ETS1/2, unlike GABPA, only activate −146C>T mutant TERT promoter through cooperation with p52 downstream of non-canonical NF-κB signaling. p52 is a member of the NF-κB family of transcription factors which regulate gene expression in response to a wide array of signaling by binding to consensus κB sites of 5′-GGGRNYYYCC-3′ (R is a purine, Y is a pyrimidine, and N is any nucleotide). The major domains of ETS1 protein include the PNT domain, the acidic transactivation domain, the ETS DNA-binding domain and autoinhibitory module which consists of inhibitory helix 1 (HI1), inhibitory helix 2 (HI2), helix 4 (H4), and helix 5 (H5). p52 consists of the Rel homology domain and the glycine-rich region.

We next determined the crystal structure of p52-RHD (residues 35–329) in complex with ETS1331–441 and a 15 bp DNA fragment of TERT promoter containing −146C>T ETS motif (designated as p52/ETS1/−146C>T). The final refined model contains the 15 bp DNA fragment, p52 residues 226–328 designated as the dimerization subdomain of p52-RHD (p52-DSD), and ETS1 residues 332–437. The DNA-binding subdomain of p52-RHD (p52-DBSD, residues 35–225) is assumed to be disordered as its electron densities are not clear enough for unambiguous model building. H3 inserts into the major groove of the DNA and contacts the GGAA central core specifically. In the p52/ETS1/−146C>T ternary complex structure, ETS1 recognizes the −146C>T TERT promoter exclusively and concurrently interacts with p52-DSD. The interaction of p52 and ETS1 buries a total solvent accessible surface area of 1187 Å2. p52 uses the loops flanking one end of the β-barrel of p52-DSD to interact with α-helices H1, H4, H5, loop H4–H5 and N-terminal region of ETS1 domain predominantly through a network of hydrogen bonds and salt bridge contacts, supplemented with additional van der Waals contacts. Structural superposition of ETS1 in the p52/ETS1/−146C>T complex and the autoinhibited ETS1 showed that p52-DSD and the HI-1 and HI-2 inhibitory helices pack against ETS1 residues 331–441 through overlapping surface regions, suggesting that the HI-1 and HI-2 inhibitory helices would interfere with the binding of ETS1 to p52-DSD. On the other hand, binding of p52 to ETS1 would displace the HI-1 and HI-2 helices, therefore counteracting the DNA binding autoinhibition of ETS1. Within the crystal lattice of the p52/ETS1/−146C>T complex, two p52-DSD molecules homodimerize through a 2-fold crystallographic symmetry. Such a p52-DSD homodimer is essentially identical to that observed in the structure of p52 homodimer in complex with the κB site, suggesting that the p52/ETS1 heterodimer can dimerize further via p52 homodimerization to form a heterotetramer.

> ADGPYLVIVEQPKQRGFRFRYGCEGPSHGGLPGASSEKGRKTYPTVKICNYEGPAKIEVDLVTHSDPPRAHAHSLVGKQCSELGICAVSVGPKDMTAQFNNLGVLHVTKKNMMGTMIQKLQRQRLRSRPQGLTEAEQRELEQEAKELKKVMDLSIVRLRFSAFLRASDGSFSLPLKPVISQPIHDSKSPGASNLKISRMDKTAGSVRGGDEVYLLCDKVQKDDIEVRFYEDDENGWQAFGDFSPTDVHKQYAIVFRTPPYHKMKIERPVTVFLQLKRKRGGDVSDSKQFTYYPLV;> GSGPIQLWQFLLELLTDKSCQSFISWTGDGWEFKLSDPDEVARRWGKRKNKPKMNYEKLSRGLRYYYDKNIIHKTAGKRYVYRFVCDLQSLLGYTPEELHAMLDVKPDADE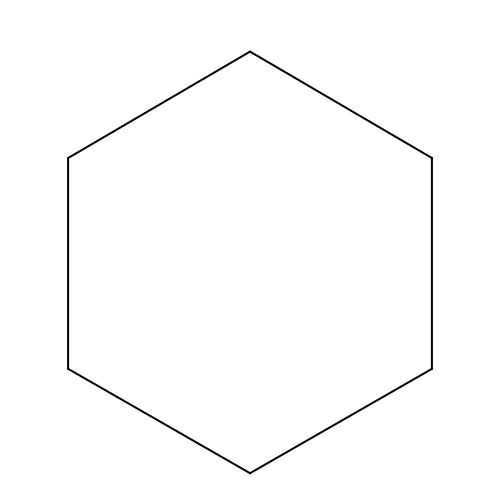CYCLOHEXANE | C6 H12 | XDTMQSROBMDMFD-UHFFFAOYSA-N(2S)-2-{[HYDROXY(4-IODOBENZYL)PHOSPHORYL]METHYL}PENTANEDIOIC 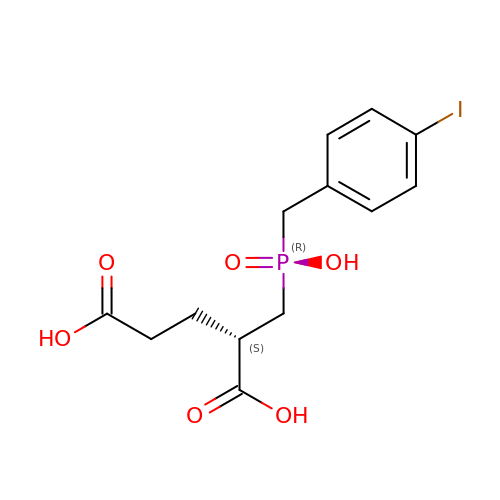ACID | C13 H16 I O6 P | PPTCQJLGUKWAEP-SNVBAGLBSA-N>[2x]VKSKAKKTVDAHSDEYKIRRERNNIAVRKSRDKAKMRNLETQHKVLELTAENERLQK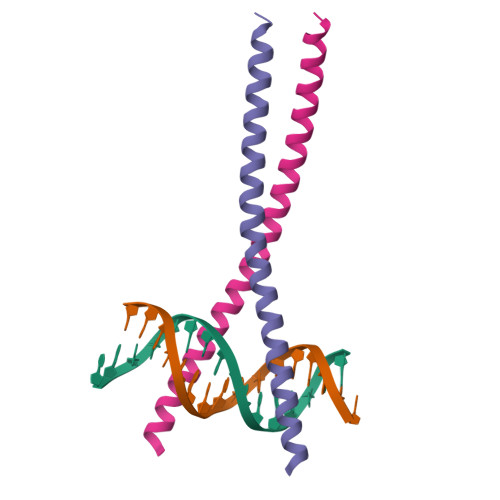KVEQLSRELSTLRNLFKQLPE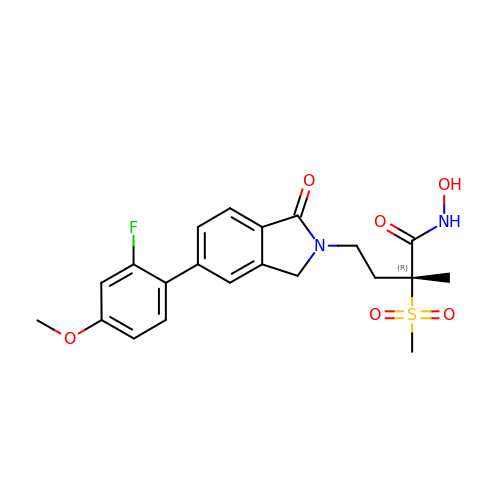(2~{R})-4-[6-(2-fluoranyl-4-methoxy-phenyl)-3-oxidanylidene-1~{H}-isoindol-2-yl]-2-methyl-2-methylsulfonyl-~{N}-oxidanyl-butanamide | C21 H23 F N2 O6 S | BYDRVBMZUCDIRW-OAQYLSRUSA-N>[3x]MIAVKDITDLNIQDIISQLTSEVINGDTTPSSAKFACEINSYIINYNLSNI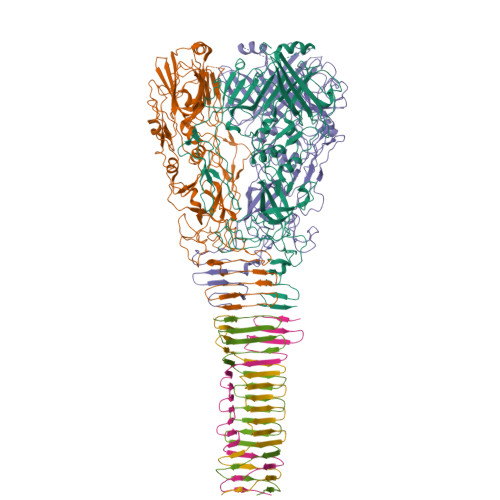NLINTQLKNTKILYRKGLISKLDYEKYKRYCIISRFKNNIDEFILYFSTNYKDSQSLKIAIKELQNSCSSSLILELPHDYIRKIDVLLTSIDSAIQRSSDLNKTIIKQLNKLRSSLSRYIGYNNVLQKQEITINIKPINKNFELEDISFVSTRNKQYFKHNSLTLKNPHIEKLEVCENIYGINGWLTFDLAYINNHKDFNFLLSPNQPILLDIQINDSFNFYKKESKKDHHKRTTRFIAIGFNSNSIDIHENFEYSIYSYTKNVSSGVKKFKIQFHDPLKALWTKHKPSYIALNKSLDDIFKDNFFFDSLFSLDTNKSNNLKIRIPQAFISTVNRNFYDFFIQQLEQNKCYLKYFCDKKSGKVSYHVVDQVDNDLQRNIVNSDEDLKDKLSPYDISCFKKQILISNKSNFYVKEKNICPDVTLNTQRKEDRKISDTLVKPFSSILKDNLQSVEYIQSNNDDKQEIITTGFEILLTSRNTLPFLDTEITLSKLDNDQNYLLGATDIKSLYISQRKLLFKRSKYCSKQLYENLHNFHYKSDSESDVYEKIAFTKYPSLTHDNSITYKIKDYSNLTPEYPKYKSFSNFYINGRITIGENVNNDSKKAYKFFKNHKPEESSIAEFQENGEKGTSAILNSKADILYAIEIAKEMLSDKSSDKPIIYLPLKVNINSANNQFIPLRNDDIILIEIQSFTKGEIIELISNSAISTKKAQQQLLQRQLLGSKENCEMAYTQTSDSETFSLTQVNEDCENSFLINDKKGIFLRYKSKGN;>MDYKDDDDKDYKDDDDKDYKDDDDKGSKADHIFNLEEQGLLIDIKDDSKGCTTKLESSGKITHNATESIESSADKQIIENVKDSKISITEKEILLATKKSSIMLSEDKIVIKIGNSLIILDDSNISLESATINIKSSANINIQASQNIDIKSLNNSIKADVNLNAEGLDVNIKGSVTASIKGSAATMVG[3x]4-({3-[(dimethylamino)methyl]-1H-indol-1-yl}methyl)-N-hydroxybenzamide 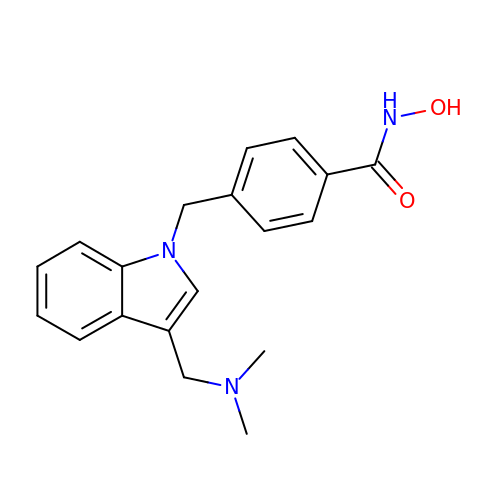| C19 H21 N3 O2 | LYCCCRFBRDLGGA-UHFFFAOYSA-N> SIESTSKSNFQKLSRGNIDVLKGRGSISSTRQRAIYPYFEAANADEQQPLFFYIKKDRFDNHGYDQYFYDNTVGPNGIPTLNTYTGEIPSDSSSLGSTYWKKYNLTNETSIIRVSNS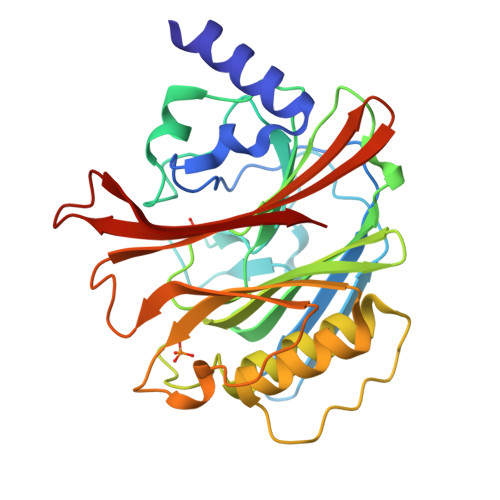ARGANGIKIALEEVQEGKPVIITSGNLSGSTTIVARKEGYIYKVHTGTTKSLAGFTSTTGVKKAVEVLELLTKEPIPRVEGIMSNDFLVDYLSENFEDSLITYSSSEKKPDSQITIIRDNVSVFPYFLDNIPEHGFGTSATVLVRVDGNVVVRSLSESYSLNADASEISVLKVFSKKF> GGGHMFDYGKRTYIMGILNVTPDSFSDGGDFNNLDIAIQHAKDMVDQGADIIDLGGESTRPGHSYVDSDEELRRVIPVIKKLKQELDIPISIDTYKADVAEEALKLGVTMVNDVWGLRKDKNMASVIGKYDAEVCIMHNQDGTN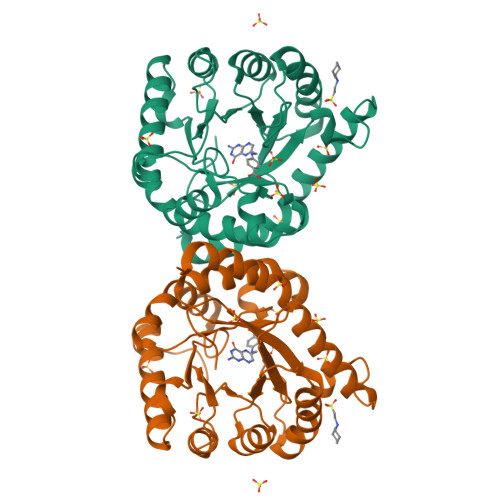YDKDIMESIKDFFKVSIEMAMSCGVKKEKIVLDPGVGFGKDFEQNIEVLRRLNELKDLGYPILLGTSRKSVIGKVLPVEPKKRLEGTIATTVLGIRDGVDIVRVHDVYENLMAARMTDAIYRK>[4x]GMTNTLKTSYQKTPYKLGGNGPRNVGVL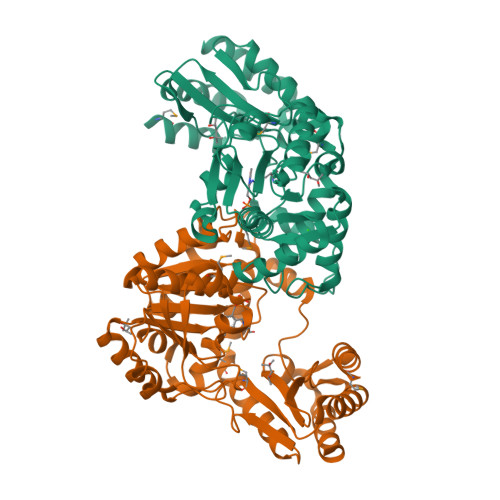TEALQNIDDNLESDIYGNGAVIEDFETKIAKILGKQSAVFFPSGTMAQQIALRIWADRKENRRVAYHPLSHLEIHEQDGLKELQQITPLLLGTANQLLTIDDIKSLREPVSSVLIELPQREIGGQLPAFEELEKISEYCHEQGISLHLDGARLWEITPFYQKSAEEICALFDSVYVSFYKGIGGIAGAILAGNDDFVQEAKIWKRRYGGDLISLYPYILSADYYFEKRIGKMAEYFEAAKGLAERFNSCSGVKTVPEVPVSNMFHVYFENSADEIGAILTKIQDETGVGISGYLQEKSADVCAFEVSVGDAFAEIPAKNLELVFRCLEKEL> ALDAAETGHTSSVQPEDVIETRYVQTSQTRDEMSLESFLGRSGCIHESKLEVTLANYNKENFTVWAINLQEMAQIRRKFELFTYTRFDSEITLVPCISALSQDIGHITMQYMYVPPGAPVPNSRDDYAWQSGTNASVFWQHGQAYPRFSLPFLSVASAYYMFYDGYDEQDQNYGTANTNNMGSLCSRIVTEKHIHKVHIMTRIYHKAKHVKAWCPRPPRALEYTRAHRTNFKIEDRSIQTAIVTRPIITTA;> RIIQITRGDSTITSQDVANAIVAYGVWPHYLSSKDASAIDKPSQPDTSSNRFYTLRSVTWSSSSKGWWWKLPDALKDMGIFGENMFYHYLGRSGYTIHVQCNASKFHQGTLIVALIPEHQIASALHGNVNVGYNYTHPGETGREVKAETRLNPDLQPTEEYWLNFDGTLLGNITIFPHQFINLRSNNSATIIAPYVNAVPMDSMRSHNNWSLVIIPICPLETSSAINTIPITISISPMCAEFSGARAKRQ;> GLPVFITPGSGQFLTTDDFQSPCALPWYHPTKEISIPGEVKNLVEICQVDSLVPINNTDTYINSENMYS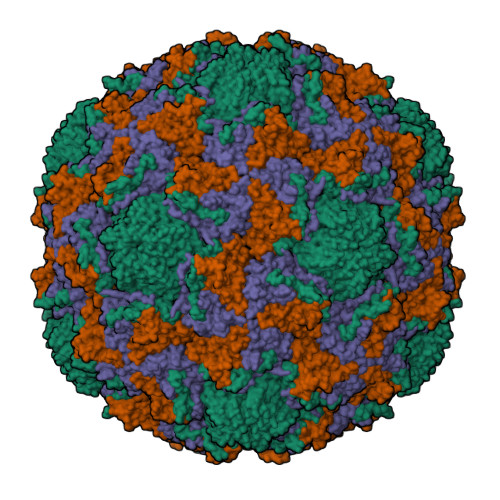VVLQSSINAPDKIFSIRTDVASQPLATTLIGEISSYFTHWTGSLRFSFMFCGTANTTVKLLLAYTPPGIAEPTTRKDAMLGTHVIWDVGLQSTISMVVPWISASHYRNTSPGRSTSGYITCWYQTRLVIPPQTPPTARLLCFVSGCKDFCLRMARDTNLHLQSGAIAQ>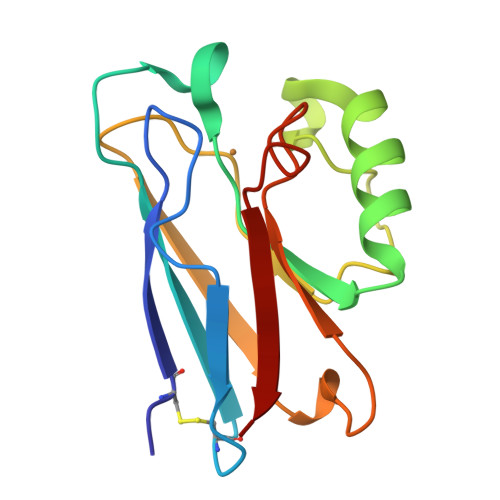AECSVDIQGNDQMQFNTNAITVDKSCKQFTVNLSHPGNLPKNVMGHNWVLSTAADMQGVVTDGMASGLDKDYLKPDDSRVIAHTKLIGSGEKDSVTFDVSKLKEGEQYMFFCAAAAHAAAAMKGTLTLK[2x]>[4x]MPYAGSELPRRPLPPAAQERDAEPRPPHGELQYLGQIQHILRCGVRKDDRTGTGTLSVFGMQARYSLRDEFPLLTTKRVFWKGVLEELLWFIKGSTNAK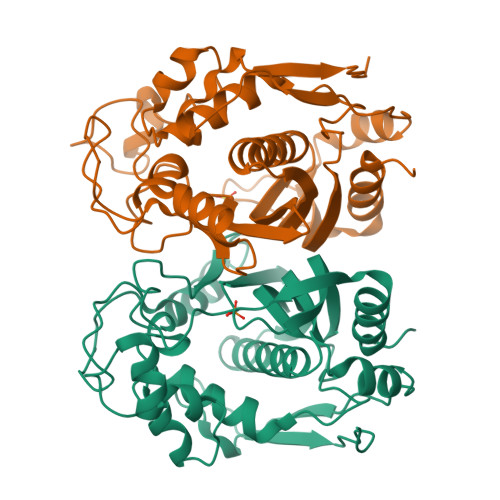ELSSKGVKIWDANGSRDFLDSLGFSTREEGDLGPVYGFQWRHFGAEYRDMESDYSGQGVDQLQRVIDTIKTNPDDRRIIMCAWNPRDLPLMALPPCHALCQFYVVNSELSCQLYQRSGDMGLGVPFNIASYALLTYMIAHITGLKPGDFIHTLGDAHIYLNHIEPLKIQLQREPRPFPKLRILRKVEKIDDFKAEDFQIEGYNPHPTIKMEMAV The systemic RNAi-defective (SID) transmembrane family member 2 (SIDT2) is a putative nucleic acid channel or transporter that plays essential roles in nucleic acid transport and lipid metabolism. Here, we report the cryo-electron microscopy (EM) structures of human SIDT2, which forms a tightly packed dimer with extensive interactions mediated by two previously uncharacterized extracellular/luminal β-strand-rich domains and the unique transmembrane domain (TMD). The TMD of each SIDT2 protomer contains eleven transmembrane helices (TMs), and no discernible nucleic acid conduction pathway has been identified within the TMD, suggesting that it may act as a transporter. Notably, SIDT2 can hydrolyze C18 ceramide into sphingosine and fatty acid with a slow rate.

As SIDT2 localizes to the plasma membrane and late endosomal and lysosomal membrane with different pH environments, Condition 1 (the apo state in pH 7.4, hereafter apoSIDT2-pH 7.4) and Condition 2 (the apo state in pH 5.5, hereafter apoSIDT2-pH 5.5) were used to investigate whether the structure of SIDT2 is affected by pH conditions. The apoSIDT2-pH 7.4, apoSIDT2-pH 5.5, and SIDT2-pH 5.5 plus miRNA structures were determined at overall resolutions of 3.16 Å, 3.21 Å, and 2.87 Å, respectively. The cytoplasmic domain (CTD) was invisible in the maps of apoSIDT2-pH 7.4 and apoSIDT2-pH 5.5, reflecting intrinsic flexibility.

>[2x]MFALGLPFLVLLVASVESHLGVLGPKNVSQKDAEFERTYVDEVNSELVNIYTFNHTVTRNRTEGVRVSVNVLNKQKGAPLLFVVRQKEAVVSFQVPLILRGMFQRKYLYQKVERTLCQPPTKNESEIQFFYVDVSTLSPVNTTYQLRVSRMDDFVLRTGEQFSFNTTAAQPQYFKYEFPEGVDSVIVKVTSNKAFPCSVISIQDVLCPVYDLDNNVAFIGMYQTMTKKAAITVQRKDFPSNSFYVVVVVKTEDQACGGSLPFYPFAEDEPVDQGHRQKTLSVLVSQAVTSEAYVSGMLFCLGIFLSFYLLTVLLACWENWRQKKKTLLVAIDRACPESGHPRVLADSFPGSSPYEGYNYGSFENVSGSTDGLVDSAGTGDLSYGYQGRSFEPVGTRPRVDSMSSVEEDDYDTLTDIDSDKNVIRTKQYLYVADLARKDKRVLRKKYQIYFWNIATIAVFYALPVVQLVITYQTVVNVTGNQDICYYNFLCAHPLGNLSAFNNILSNLGYILLGLLFLLIILQREINHNRALLRNDLCALECGIPKHFGLFYAMGTALMMEGLLSACYHVCPNYTNFQFDTSFMYMIAGLCMLKLYQKRHPDINASAYSAYACLAIVIFFSVLGVVFGKGNTAFWIVFSIIHIIATLLLSTQLYYMGRWKLDSGIFRRILHVLYTDCIRQCSGPLYVDRMVLLVMGNVINWSLAAYGLIMRPNDFASYLLAIGICNLLLYFAFYIIMKLRSGERIKLIPLLCIVCTSVVWGFALFFFFQGLSTWQKTPAESREHNRDCILLDFFDDHDIWHFLSSIAMFGSFLVLLTLDDDLDTVQRDKIYVF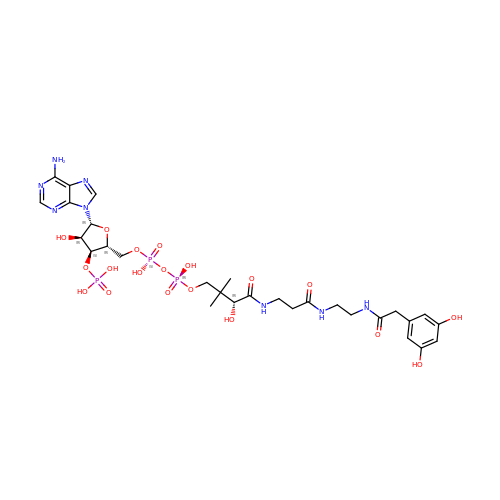[(2R,3S,4R,5R)-5-(6-AMINO-9H-PURIN-9-YL)-4-HYDROXY-3-(PHOSPHONOOXY)TETRAHYDROFURAN-2-YL]METHYL (3R)-4-({3-[(2-{[(3,5-DIHYDROXYPHENYL)ACETYL]AMINO}ETHYL)AMINO]-3-OXOPROPYL}AMINO)-3-HYDROXY-2,2-DIMETHYL-4-OXOBUTYL DIHYDROGEN DIPHOSPHATE | C29 H43 N8 O19 P3 | MSJGSRHUBFYIJV-CECATXLMSA-N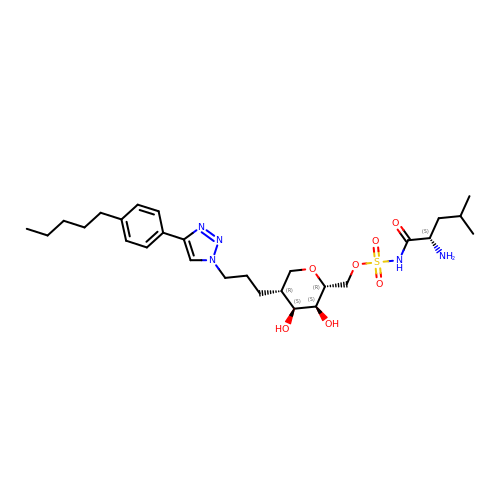[(2~{R},3~{S},4~{S},5~{R})-3,4-bis(oxidanyl)-5-[3-[4-(4-pentylphenyl)-1,2,3-triazol-1-yl]propyl]oxan-2-yl]methyl ~{N}-[(2~{S})-2-azanyl-4-methyl-pentanoyl]sulfamate | C28 H45 N5 O7 S | APPGUXVTRIHQDP-GVPWJHIJSA-N>[2x]MAAATGPSFWLGNETLKVPLALFALNRQRLCERLRKNPAVQAGSIVVLQGGEETQRYCTDTGVLFRQESFFHWAFGVTEPGCYGVIDVDTGKSTLFVPRLPASHATWMGKIHSKEHFKEKYAVDDVQYVDEIASVLTSQKPSVLLTLRGVNTDSGSVCREASFDGISKFEVNNTILHPEIVECRVFK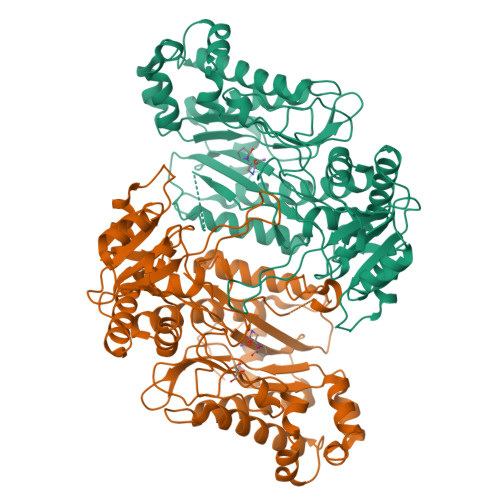TDMELEVLRYTNKISSEAHREVMKAVKVGMKEYELESLFEHYCYSRGGMRHSSYTCICGSGENSAVLHYGHAGAPNDRTIQNGDMCLFDMGGEYYCFASDITCSFPANGKFTADQKAVYEAVLRSSRAVMGAMKPGVWWPDMHRLADRIHLEELAHMGILSGSVDAMVQAHLGAVFMPHGLGHFLGIDVHDVGGYPEGVERIDEPGLRSLRTARHLQPGMVLTVEPGIYFIDHLLDEALADPARASFLNREVLQRFRGFGRVRIEEDVVVTDSGIELLTCVPRTVEEIEACMAGCDKAFTPFSGPK> MTIDDSNRLLMDVDQFDFLDDGTAQLSNNKTDEEEQLYKRDPVSGAILVPMTVNDQPIEKNGDKMPLKFKLGPLSYQNMAFITAKDKYKLYPVRIPRLDTSKEFSAYVSGLFEIYRDLGDDRVFNVPTIGVVNSNFAKEHNATVNLAMEAILNELEVFIGRVKDQDGRVNRFYELEESLTVLNCLRTMYFILDGQDVEENRSEFIESLLNWINRSDGEPDEEYIEQVFSVKDSTAGKKVFETQYFWKLLNQLVLRGLLSQAIGCIERSDLLPYLSDTCAVSFDAVSDSIELLKQYPKDSSSTFREWKNLVLKLSQAFGSSATDISGELRDYIEDFLLVIGGNQRKILQYSRTWYESFCGFLLYYIPSLELSAEYLQMSLEANVVDITNDWEQPCVDIISGKIHSILPVMESLDSCTAAFTAMICEAKGLIENIFEGEKNSDDYSNEDNEMLEDLFSYRNGMASYMLNSFAFELCSLGDKELWPVAIGLIALSATGTRSAKKMVIAELLPHYPFVTNDDIEWMLSICVEWRLPEIAKEIYTTLGNQMLSAHNIIESIANFSRAGKYELVKSYSWL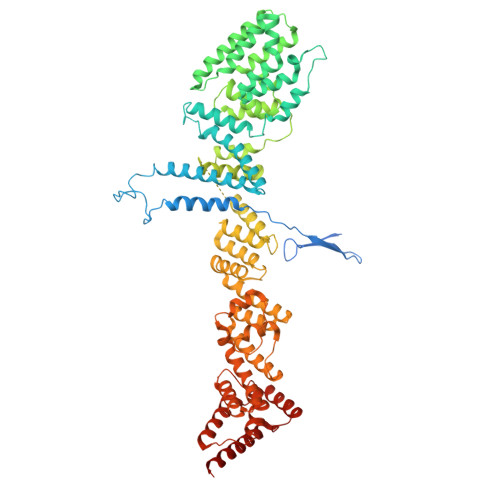LFEASCMEGQKLDDPVLNAIVSKNSPAEDDVIIPQDILDCVVTNSMRQTLAPYAVLSQFYELRDREDWGQALRLLLLLIEFPYLPKHYLVLLVAKFLYPIFLLDDKKLMDEDSVATVIEVIETKWDDADEKSSNLYETIIEADKSLPSSMATLLKNLRKKLNFKLCQAFM>[3x]AEIYNKDGNKVDLYGKAVGLHYFSKGNGENSYGGNGDMTYARLGFKGETQINSDLTG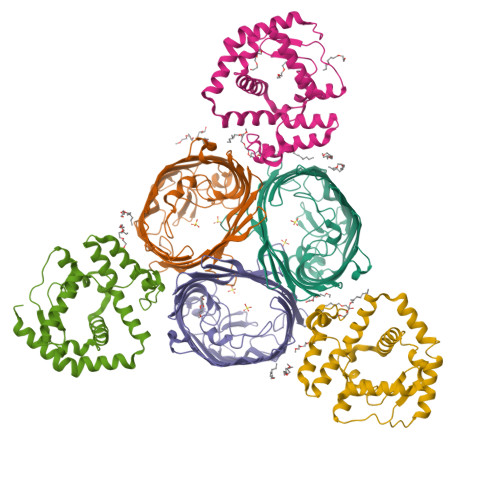YGQWEYNFQGNNSEGADAQTGNKTRLAFAGLKYADVGSFDYGRNYGVVYDALGYTDMLPEFGGDTAYSDDFFVGRVGGVATYRNSNFFGLVDGLNFAVQYLGKNERDTARRSNGDGVGGSISYEYEGFGIVGAYGAADRTNLQEAQPLGNGKKAEQWATGLKYDANNIYLAANYGETRNATPITNKFTNTSGFANKTQDVLLVAQYQFDFGLRPSIAYTKSKAKDVEGIGDVDLVNYFEVGATYYFNKNMSTYVDYIINQIDSDNKLGVGSDDTVAVGIVYQF;>[3x]CASSSSGDRPQGRSDPLEGFNRTMFNFNFNVVDPYVLRPVAVAWRDYVPQPARNGLSNFTSNLEEPAVMVNYFLQGDPYKGMVHFTRFFLNTILGMGGLIDVAGMANPQLQRVEPHRFGSTLGHYGVGYGPYVQLPFYGSFTLRDEGGDMADGLYPVLSWLTWPMSIGKWAVEGIETRAQLLDSDGLLRQSSDPYILMREAYFQRHDFIANGGKLTPADNPNAQAIQDELKDIDSQ> MGLLSLIRGLKKKEGEARILVLGLDNAGKTTILKALSEEDITT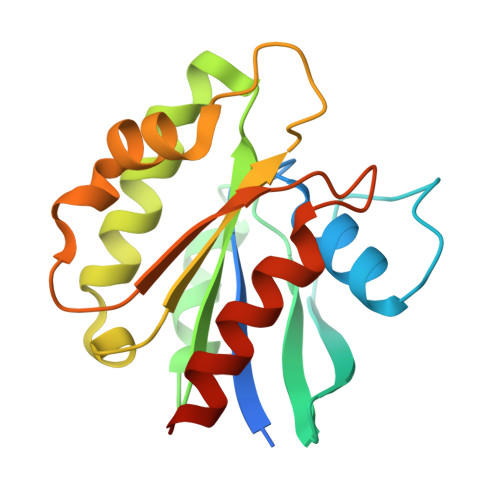ITPTQGFNIKSLSRDGFNLKIWDIGGQKSIRPYWRNYFDQTDALIYVIDSADSKRLSESEFELTELLQEEKMTGVPLLVFANKQDLVGALAADEIASTLDLTSIRDRPWQIQACSAKQGTGLKEGMEWMMKQVKLEHHHHHH> AVTVVPDPTCCGTLSFKVPKDAKKGKHLGTFDIRQAIMDYGGLHSQEWCAKGIVNPTFTVRMHAPRNAFAGLSIACTFDDYKRIDLPALGNECPPSEMFELPTKVFMLKDADVHEWQFNYGELTGHGLCNWANVATQPTLYFFVASTNQVTMAADWQCIVTMHVDMGPVIDRFELNPTMTWPIQLGDTFAIDRYYEAKEIKLDGSTSMLSISYNFGGPVKHSKKHAISYSRAVMSRNLGWSGTISGSVKSVSSLFCTASFVIFPWECEAPPTLRQVLWGPHQIMHGDGQFEIAIKTRLHSAATTEEGFGRLGILPLSGPIAPDAHVGSYEFIVHINTWRPDSQVHPPMFSSSELYNWFTLTNLKPDANTGVVNFDIPGYIHDFASKDATVTLASNPLSWLVAATGWHYGEVDLCISWSRSKQAQAQEGSVSITTNYRDWGAYW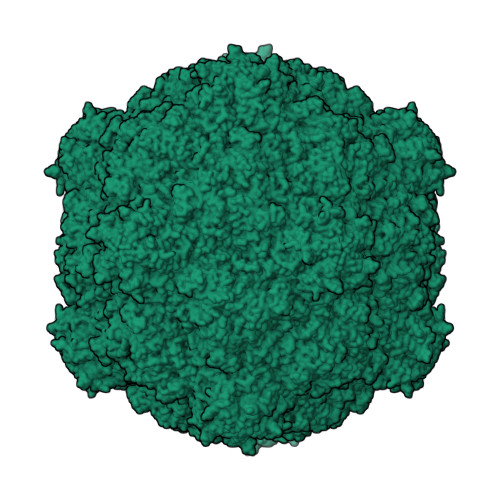QGQARIYDLRRTEAEIPIFLGSYAGATPSGALGKQNYVRISIVNAKDIVALRVCLRPKSIKFWGRSATLF> GMDFLTSTLLSGILYDGFKNGVAITTGFLKEK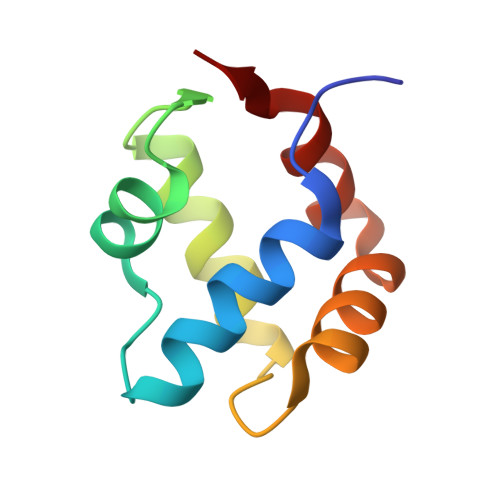LHGWIVDDTLLETLAYKVNTLELKDYGEHVIERKLNESSEIQQILKLIQPE> MATVTSVPGVYIEEDASPAMSVSASATAVPLFVARFTPLKPELAGVITRIGSWLDYTILFDSNVPSSARVTVSSTAVEPSPEFDALETASSKATTTYTYQIDDTEVVDPTASVALRLYFQNGGGPCYLYPLEKADDNGPLAALPDLIDEVGEITLLASPDPDETYRTAVYGALAASLDQHKGYFLLADSVNGDAPSAVGGSAQVAVYYPNVEVPHTRKLDDAEVAIDGYLDDEGKAVTTLAALRVVNTEFAGEIAQSLSGDLSAPLSLPPSALIAGVYGKTDGERGVWKAPANVVLNGVSDVSVRVTNEQQAELNPKGINVIRHFSDRGLVVWGSRTQKDDDDWRYIPVRRLFDAAERDIKKALQPMVFEPNSQLTWKRVQTAIDNYLYR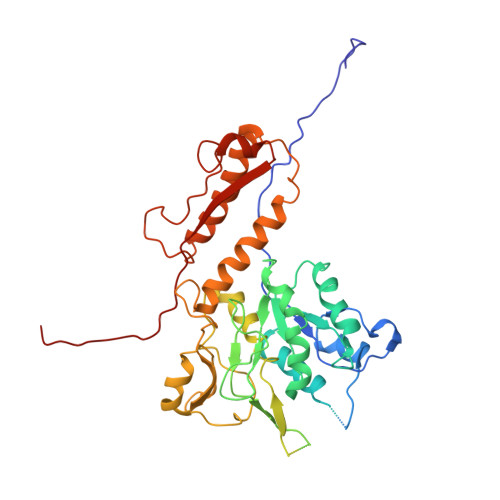LWQQGALAGNKAEEAYFVRVGKGITMTQDEINQGKMIIQVGMAAVRPAEFIILKFTQDMSQ> GHMSMQGPRTRPRKPIRAGEVLFAVGGWASGDAISSVERYDPQTNEWRMVASMSKRRCGVGVSVLDDLLYAVGGHDGSSYLNSVERYDPKTNQWSSDVAPTSTARTSVGVAVLGGFLYAVGGQDGVSALNIVERYDPKENKWTRVASMSTRRLGVAVAVLGGFLYAVGGSDGT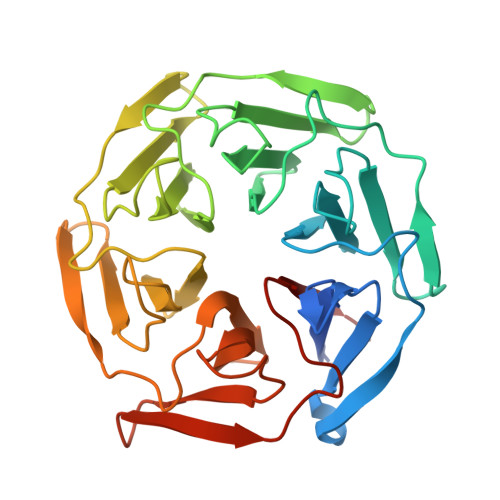SPLNTVERYNPEENRWHTIAPMGTRRKHLGCAVYQDMIYAVGGRDDTTELSSAERYNPRTNQWSPVVAMTSRRSGVGLAVVNGQLMAVGGFDGTTYLKTIEVFDPDANTWRLYGGMNYRRLGGGVGVIKMTHAE>[10x]DLTKNEKGRLTPITKQQSANSAKLTAYGTLKSALEKFQTANTALNKADLFKSTVASSTTEDLKVSTTAGAAAGTYKINVTQLAAAQSLATKTTFATTKEQLGDTSVTSRTIKIEQPGRKEPLEIKLDKGDTSMEAIRDAINDADSGIAASIVKVKENEFQLVLTANSGTDNTMKITVEGDTKLNDLLAYDSTTNTGNMQELVKAENAKLNVNGIDIERQSNTVTDAPQGITLTLTKKVTDATVTVTKDDTKAKEAIKSWVDAYNSLVDTFSSLTKYTAVEPGEEASDKNGALLGDSVVRTIQTGIRAQFANSGSNSAFKTMAEIGITQDGTSGKLKIDDDKLTKVLKDNTAAARELLVGDGKETGITTKIATEVKSYLADDGIIDNAQDNVNATLKSLTKQYLSVSNSIDETVARYKAQFTQ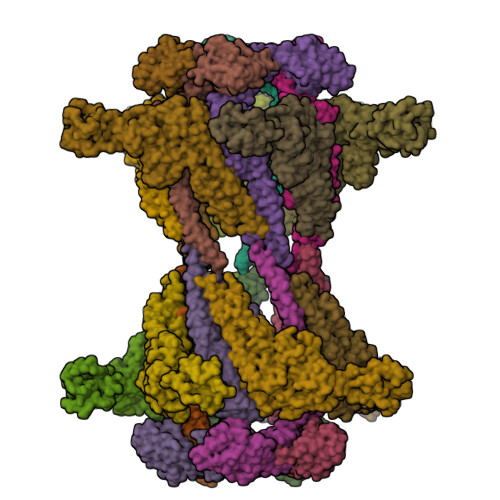LDTMMSKL;>FTANIKGLTQASRNANDGISIAQTTEGALNEINNNLQRVRELAVQSANSTNSQSDLDSIQAEITQRLNEIDRVSGQTQFNGVKVLAQDNTLTIQVGANDGETIDIDLKQINSQTLGLDTLNVQQKYKVSDTAATVTGYADTTIALDNSTFKASATGLGGTDQKIDGDLKFDDTTGKYYAKVTVTGGTGKDGYYEVSVDKTNGEVTLAGGATSPLTGGLPATATEDVKNVQVANADLTEAKAALTAAGVTGTASVVKMSYTDNNGKTIDGGLAVKVGDDYYSATQNKDGSISINTTKYTADDGTSKTALNKLGGADGKTEVVSIGGKTYAASKAEGHNFKAQPDLAEAAATTTENPLQKIDAALAQVDTLRSDLGAVQNRFNSAITNLGNTVNNLTSARSRI[10x]The Oag polymer chains are neither all of the same length nor of random length, and fall in a defined range termed the modal distribution. This distribution is regulated by two Wzz proteins in S. flexneri: WzzBSF, which confers an average modal chain-length of 10–17 Oag repeat units (short (S)-type), and WzzpHS2, which confers a very long (VL-type) modal chain-length of > 90 Oag repeat units. The S. flexneri Wzz proteins are members of the PCP1a family and are located in the inner membrane. They contain a hydrophilic periplasmic polypeptide segment, and two trans-membrane (TM) regions at the N- and C-terminal ends.

Despite low sequence similarities between PCP1a family proteins, the individual protomers have a comparable three-dimensional architecture, and self-assemble into a bell-shaped quaternary structure. However, different oligomeric sizes have been reported for different PCP1a family proteins. The crystal structure of the periplasmic domain of WzzBSF has recently been shown to form an open trimer, while chimeric hybrid protein variants based on WzzBSF and WzzBST instead formed octameric barrels. Binding analyses reveal positive cooperativity for the interaction of very-short (VS) core-plus-Oag polysaccharide (COPS) with the periplasmic domain of WzzBSF, and a decreased COPS-binding affinity for the A107P mutant. The crystal structure of the mutant protein shows only subtle structural differences near the mutation, compared to the wild-type protein.

>[3x]SNAEKWTSTAIITQPDVGQIAGYNNAMNVIYGQAAPKVSDLQETLIGRFSSAFSALAETLDNQEEPEKLTIEPSVKNQQLPLTVSYVGQTAEGAQMKLAQYIQQVDDKVNQELEKDLKDNIALGRKNLQDSLRTQEVVAQEQKDLRIRQIQEALQYANQAQVTKPQVQQTEDVTQDTLFLLGSEALESMIKHEATRPLVFSPNYYQTRQNLLDIEKLKFDDLDIHAYRYVMKPTLPIRRDSPK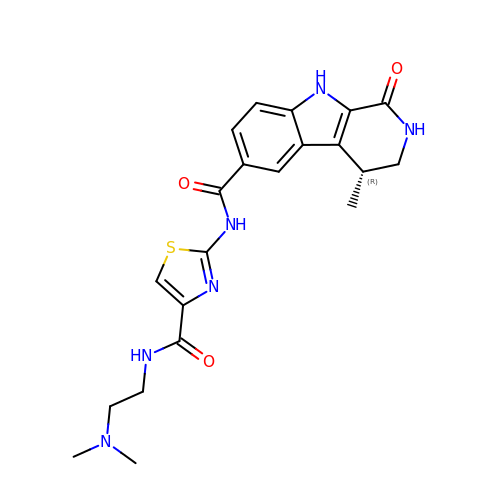(4R)-N-[4-({[2-(DIMETHYLAMINO)ETHYL]AMINO}CARBONYL)-1,3-THIAZOL-2-YL]-4-METHYL-1-OXO-2,3,4,9-TETRAHYDRO-1H-BETA-CARBOLINE-6-CARBOXAMIDE | C21 H24 N6 O3 S | QWFFPYQWUWLDBV-NSHDSACASA-N>[3x]MLYEEDYKLALEAFKKVFNALTHYGAKQAFRSRARDLVEEIYNSGFIPTFFYIISKAELNSDSLDSLISLFSSDNAILRGSDENVSYSAYLFIILYYLIKRGIIEQKFLIQALRCEKTRLDLIDKLYNLAPIISAKIRTYLLAIKRLSEALIEAR;>MPYYAFAEPFFIHAITHLHVGSGSSVEEEIALPFQRDELGYPTIYASSLKGAIKSFLLKEFPDKRDVIYKVLGEDENPEEASLGTFLDAILFAIPSRIIEIDSAKPYVWVYVTTYELLKKVKLYLDSISQLSNASFSNLKNKIDTILAKEGKNITLDSDLKSAILNEDFYVELEALNNKIPSIINAGVPLLVLEDSIGREVINRSLIRVRRIRIDRDKKVVETGGLWSEEYVPMKTIFFSVLLGKESKESAIFASCILRNLRYVILGGKETIGKGIVELRWVKDVI[4x];> MKRVL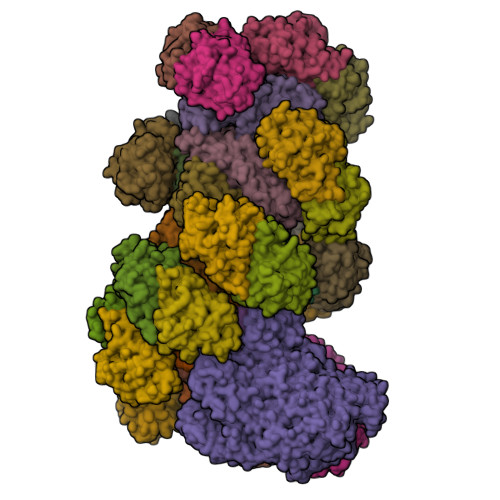IKPLEPLMFRSQGEFEPLITGSHTAAQSLIIPRPSTIAGMLGYILFNKSSGTGDWLSDLTNLLATIYGTFIETNGEYLFPLRMGNHLALVDQQHLINLPTLLEKEYERREKGIYELFYDKNKLFQIINHQDRIGISIDKSTRTVKEHYLYSARYLAFKKEVNYVIFIDNDAISDKINGKIVNFGGENRIAKLEVDDYKVDTSIEEEYYLALSPILIPDEALDNFLDNISDYVAMGKVDKISLGFDIANTKRKEMLTAILEGSIVKRSIIDFIKNEIKNDLRYRFSKYEKIGYNTLMSLCKLALRKILS;> MAIDFLVNILELIKEKQCNINLFSAISLTSIVYNNFGEFLSNNQSYSTNNPLLKYHIIILNDKNKTKDVEEKRNIFKREVAELISRNFKLDGEKVRNYFDSLKEVLKSLKYTIVDVEITTRTRALIGVSTSLGKLIFGSGISFDPYMNLPYIPASEIKGIVRSYIEGKLGEQEAEEIFGNEEREGNVNFTDAYPTRSKDFLFVPDVITPHYNGKKSEADAEPRPVIHLTIAPKVTFRFLIYYKREDVGKPICDSMPIILIRGLGARSSVGYSLFELRKIEVIKAAAHHHHHHHHHH;> MEELLMSLKLKALYPLTGGYNRHSINPFYEELVRPTEIKGLWRWWNRVLFNTLAYSTKGKLYTYESIDRLFEDVFGSENKKSAVRLEVITDEGNDNRFELSYVELDKVIDCLRNYKRKVSLDFIDNTLIAEIEGSTKIPISFKSNLDIDKIIKDLVHNNKLLSFELLGFKSVEIDATKISDKKILKEILRDLITNYLEYFNIKQEVTFTLNIYLDKSREHKQNFEDKLKFALYSLLVFILLGGIGRKTSRGFGSLSIIDVKCYDNSICKKIEDLAKNFLKISSGNELKSKIESILDCIKNSCIDTLYIENNILSEIDPKKNVVYFINSDLFEVKRINDKEKVLANIYKAVSSEGCCIKSIITDKYVRKSFLIAFGGYRKVEKDKGLDIGFIKNYLCETCETVSSFNIVDFLLSEGSFMSDYILQYEHRNSLLRFKLISDNSNNSYLIGYILHSSYFKKIDIKYVRCILEKLTYCVI;> MSIDNVLREFLDYKIIALLHDPPNKAWVITGRARNLTQQLSNIRASRKHEKVAKYIINQLFGKNYSEKVDNADKLASSIDRYLGSIVYKERSLFENRSIFLKNILLSNIQRDIGNLFPKDKSKLDNLILEYKKLLNVINKTNLILKYQLFYLIYELVWIDSKYENTPSDTRNPTHTIFDHLYATAAMMNWILSLEKEAKGYLLGIDTIGVADFISKGRKTRDLWISSYLVSALLWYVITWFIEEYGPDVILFPSLRFNQFYAFYLLEKLRKEGVSEDVIDEIKELITKYIFNGDDLFENLKIPPYPIIPGRITLILPGLIREGEEYKKVQDDNCFISKVKERYNEGWRKLIEGLRCYSERKREDGFWNLVCRVLKLTEDLLQTTPLNIRVKQVSVTEDEIFNNNKLRSDSWKIYDNKYRQLVSEFKKSKLVKVTPESRLKLFELTKFDKLPQIGEKSKRGYEFCTSCGVLPAVVIMPKEDELEKKLIDLGIARDEKDVRSIKNMISPGERLCPWCLVKRALGAEPRLMRILLLGDLYSVEKIVNEIVSRDVKIEIPSTSDIASIKTFEEMIEKKNEICEDLKEEEVCEKPSESVLSMWQWFNKNYYNGINLTIDPEEYWFSEKRRRYYFSVFRRHRITFPSPYYALVRADSDYLGDLLEGKLTPYLAGIIDSGDYANISEKKEEVNKLLEEYLVNAGSGSIVDYVKTVLKCIRENLNKCSCAEKIYSNEVAKVMFRVNVEKANVEEEVKNSLEYFETILNEGRIIVTPAWHVSISSALNRGLLVELELVNKHKGFVIYAGGDDLLAMLPVDEVLDFIKESRRAFAGFGTEKLGNMCLENGFVRINNAYYPSLPIVGRSYSVIIAHYADPLFFVINDSYNLLEEGKEIIRYRVMYNGEYKDAKKDVAIFRYQGLTSVIPLSLKRPIVSSVSDFNEIASIIDVILELKKRIDEGRISVSLLYDYEKYKHLIVASDEKYLTEFLVKDWIKRNSLRKHVEFTIDEKLYGVRLTIENYPIKIPNDLISNIVYTLRIIYGGEK;>[22x]MSTQREYVFIPITNSITIDVKITIGGSDHITNIDERGIHNVLVITGYAVDEKNGRLVPTLDPCDYVKGILVAGTPQQAQSNDFLTLKLPANKLYLIRKKGNISDDLKIYIPYSSPDARNSMKTKPVSISDDTIVNNIIKEVFDKIYNITQKEKVKIEKVKEDIKELFSYYALEQ>[2x]MKVTKSEIVISAVKPEQYPEGGLPEIALAGRSNVGKSSFINSLI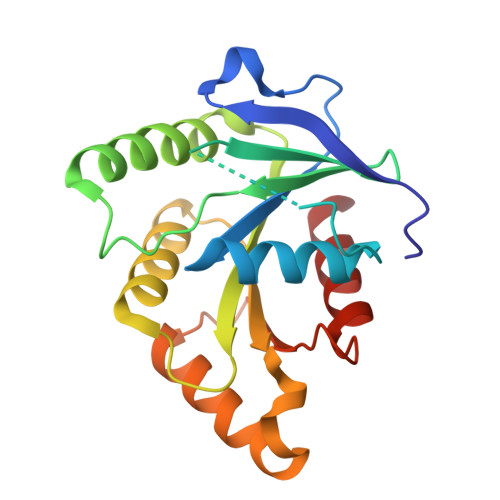NRKNLARTSSKPGKTQTLNFYIINDELHFVDVPGYGFAKVSKSEREAWGRMIETYITTREELKAVVQIVDLRHAPSNDDVQMYEFLKYYGIPVIVIATKADKIPKGKWDKHAKVVRQTLNIDPEDELILFSSETKKGKDEAWGAIKKMINR> MVAGAVAGALIGAAVVAATAATGGLAAVILAGSIAAGGLSMFQIVKGLTTIFELPEPTTGVLIRGS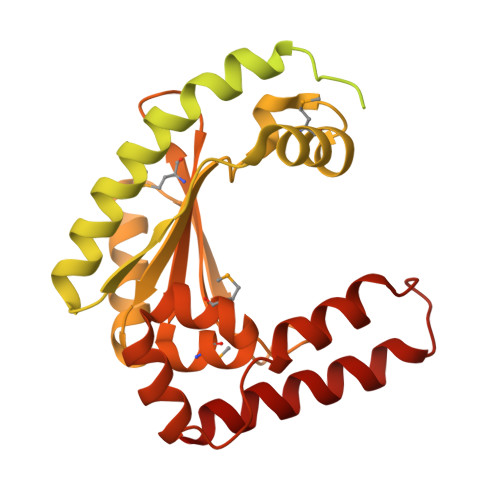FNVYVNSRNAMRAGDDVSATCSGLPLNHPLWPFPVLIAEGSATVYINGKPAARLQSKMVCGAHIKTGSQNTFIGGPTERVAFVLDLEEWLHTGLEALGLAALAGGLLLAAMAGVAALVGVVAIGGLMMGGMALLGDLGDRLGPGYRDLFQGVAGMALLGFGPKMARLGNAPKGAPKTQVPKGFEKVYGKAPAAKAEIDAVADGLAAKHGGRVAKAPIKSRERAMQKINNDYKGDPTKIKDLARNTIIVEGDKVNTVAAELANRGAKVKVIDGNADPLGYSGVNSTMNTKAGIPGEIQVNSPEMIYAKESEDMARILLGNDTYDAVAAKAGVPGGQGHKYYEDWRVLDPKSPEAQAIAEKSRAYYDAVRKGNGN>SNADEVQVAVAANFTAPIQAIAKEFEKDTGHRLVAAYGATGQFYTQIKNGAPFQVFLSADDSTPAKLEQEGEVVPGSRFTYAIGTLALWSPKAGYVDAEGEVLKSGSFRHLSIANPKTAPYGLAATQAMDKLGLAATLGPKLVEGQNISQAYQFVSSGNAELGFVALSQIYKDGKVATGSAWIVPTELHDPIRQDAVILNKGKDNAAAKALVDYLKGAKAAALIKSYGYEL[2x]

Acquisition of the trace-element molybdenum via the high-affinity ATP-binding cassette permease ModABC is essential for Pseudomonas aeruginosa respiration in anaerobic and microaerophilic environments. Molybdenum, which predominantly occurs as the oxyanion molybdate (MoO42−; henceforth MoO), is imported via the high-affinity ATP-binding cassette (ABC) permease, ModABC in P. aeruginosa. Pseudomonas aeruginosa PAO1 ModA has a non-contiguous dual-hinged bilobal structure with a single metal-binding site positioned between the two domains.

Metal binding results in a 22° relative rotation of the two lobes with the oxyanions coordinated by four residues, that contribute six hydrogen bonds, distinct from ModA orthologues that feature an additional oxyanion-binding residue. In this study, we investigated the interaction of P. aeruginosa ModA with oxyanions of the group 6 elements: Cr, Mo, and W. By combining biochemical, structural, and molecular dynamic analyses of ModA-metal complexes, we show that the SBP is permissive for binding all three oxyanions at the primary metal-binding site. Despite E. coli ModA having a high affinity for MoO (Kd = ~5–67 nM; Rech et al., 1996; Imperial et al., 1998; Ge et al., 2020), it has been shown to be permissive for binding to tungstate (WO42−; henceforth WO), the oxyanion form of tungsten (W), a group 6 element with similar chemistry to molybdenum. In P. aeruginosa, exposure to WO reduced MoO acquisition, which was attributed to competition between the two metal ions for the ModA SBP and the inappropriate sensing of W by ModE, thereby leading to repression of the modABC operon. The result was a depletion in cellular Mo, with concomitant impacts on nitrate reductase activity and inhibition of anaerobic growth in WO-supplemented media.>QSGNPFSGRTLLVNSDYSSKLDQTRQAFLSRGDQTNAAKVKYVQEKVGTFYWISNIFLLRDIDVAIQNARAAKARGENPIVGLVLYNLPDRDCSAGESSGELKLSQNGLNRYKNEYVNPFAQKLKAASDVQFAVILEPDAIGNMVTGTSAFCRNARGPQQEAIGYAISQLQASHIHLYLDVANGGWLGWADKLEPTAQEVATILQKAGNNAKIRGFSSNVSNYNPYSTSNPPPYTSGSPSPDESRYATNIANAMRQR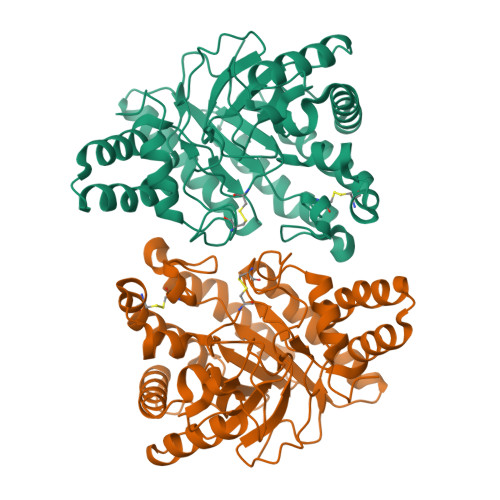GLPTQFIIDQSRVALSGARSEWGQWCNVNPAGFGQPFTTNTNNPNVDAIVWVKPGGESDGQCGMGGAPAAGMWFDAYAQMLTQNAHDEIAR[2x]> MAHHHHHHMARIPPLVVCGPSGVGKGTLIKKVLSEFPSRFRFSISCTTRNKREKETNGVDYYFVDKDDFERKLKEGQFLEFDKYANNFYGTLKSEYDLAVGEGKICLFEMNINGVKQLKESKHI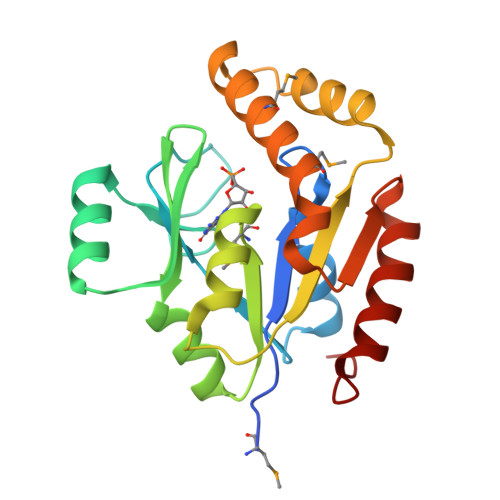QDGIYIFVKPPSIDILLGRLKNRNTEKPEEINKRMQELTREMDEADKVGFNYFIVNDDLARTYAELREYLLGSYPQLRGG> MTLQQEIIQALGAKPHINPEEEIRRSVDFLKAYLKTYPFLKS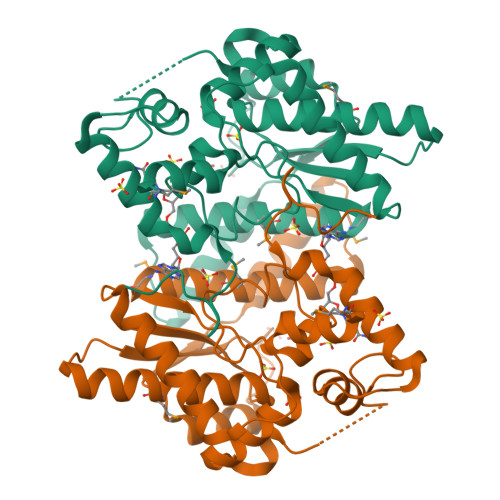LVLGISGGQDSTLAGKLSQMAIAELREETGDNALQFIAVRLPYGVQADEQDCQDAIAFIQPDRVLTVNIKGAVLASEQALREAGIELSDFVRGNEKARERMKAQYSIAGMTHGVVVGTDHAAEAITGFFTKYGDGGTDINPLHRLNKRQGKQLLAALGCPEHLYKKVPTADLEDDRPSLPDEAALGVTYDNIDDYLEGKTLDPAIAKTIEGWYVKTEHKRRLPITVFDDFWKR> MHHHHHHSAEQIMRDRSELARKGIARGRSVVVLTFRDGVLFVAENPSTALHKVSELYDRLGFAAVGKYNEFEN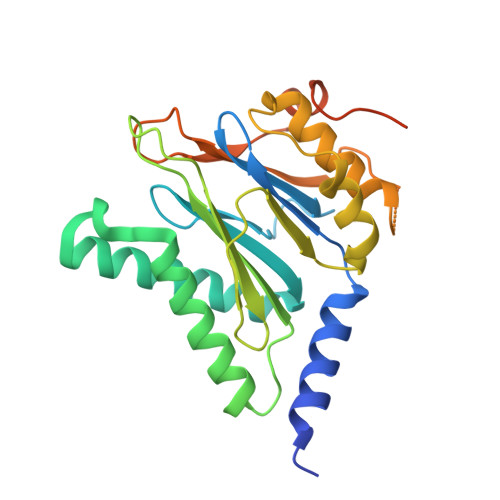LRRAGIVHADMRGYSYDRRDVTGRSLANAYAQTLGTIFTEQPKPYEVEICVAEVGRVGSPKAPQLYRITYDGSIVDEQHFVVMGGTTEPIATAMRESYRADLDLEAAVGIAVNALRQGGAGEGEKRNVDVASLEVAVLDQSRPRRAFRRIAGTALEQLVPAEPAAASESAPEPKPDTETKPADTQD> MEYEDLELITIWPSPTKNKLCQFIKQNLSKEHVVTQLFFIDATSSFPLSQFQKLVPPTLPENVRIYENIRINTCLDLEELSAITVKLLQILSMNKINAQRGTEDAVTEPLKIILYINGLEVMFRNSQFKSSPQRSHELLRDTLLKLRVMGNDENENASIRTLLEFPKEQLLDYYLKKNNNTRTSSVRSKRRRIKNGDSLAEYIWKYYADSLFE;> GSHMEVLKNIRIYPLSNFITSTKNYINLPNELRNLISEEQESKLGFLHIIESDFKPSVALQKLVNCTTGDEKILIIDIVSIWSQQKQRQHGAIYMNSLSCINITGLIVFLELLYDSPMDALRRCQVDNFNFQLRGIVIDNLSFLNFESDKNYDVINLSKFEKLFKILRKLREFLGCWIITKSFPTDFYNGIENTLVDKWSIKRKSGVTLYP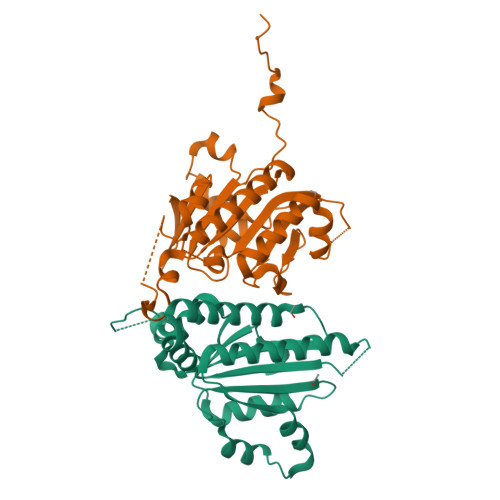TKLPDSYMKGMDLIIYREVVDGRPQYRRIAALEE>[4x]MTKNPRNNKPKKILDSSYKSKTIWQNYIDALFETFPQLEISEVWAKWDGGNVTKDGGDAKLTANIRTGEHFLKAREAHIVDP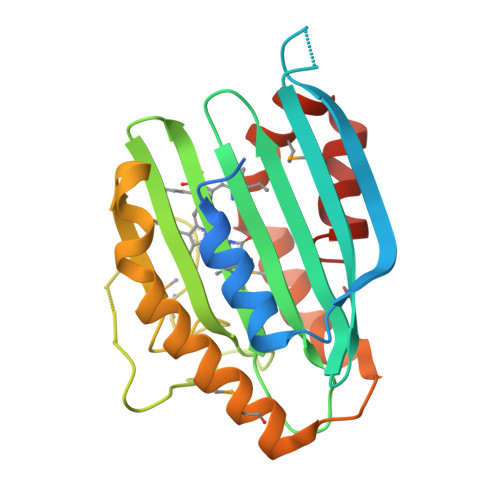NSDIYNTILYPKTGADLPCFGMDLMKFSDKKVIIVFDFQHPREKYLFSVDGLPEDDGKYRFFEMGNHFSKNIFVRYCKPDEVDQYLDTFKLYLTKYKEMIDNNKPVGEDTTVYSDFDTYMTELDPVRGYMKNKFGEGRSEAFVNDFLFSYK(3S)-N-(4'-carbamoyl[1,1'-biphenyl]-3-yl)-1-[4-(4-methylpiperazin-1-yl)pyridine-2-carbonyl]piperidine-3-carboxamide | C30 H34 N6 O3 | 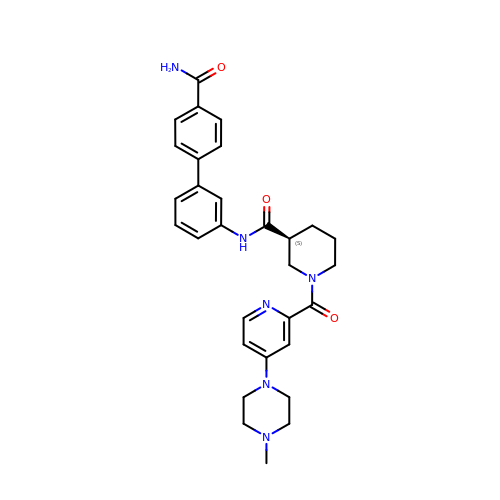KDJWESNUVQMZGH-DEOSSOPVSA-N> SDKIIHLTDDSFDTDVLKADGAILVDFWAEWCGPCKMIAPILDEIADEYQGKLTVAKLNIDQNPGTAPKY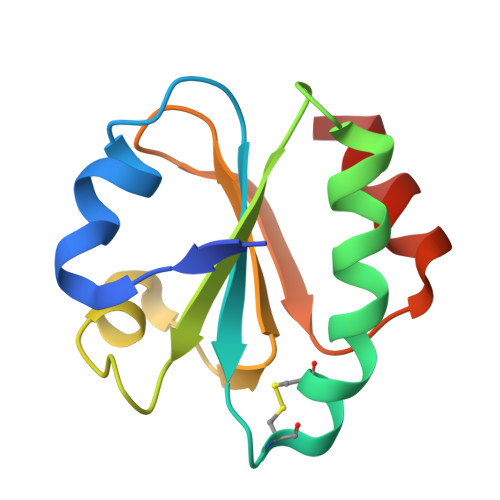GIRGIPTLLLFKNGEVAATKVGALSKGQLKEFLDANLA> MEEPEEPADSGQSLVPVYIYSPEYVSMCDSLAKIPKRASMVHSLIEAYALHKQMRIVKPKVASMEEMATFHTDAYLQHLQKVSQEGDDDHPDSIEYGLGYDCPATEGIFDYAAAIGGATI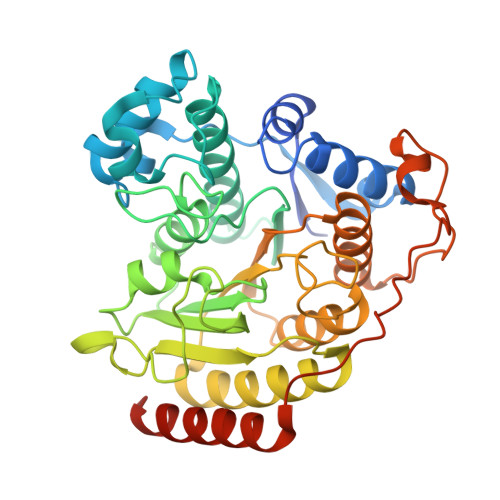TAAQCLIDGMCKVAINWSGGWHHAKKDEASGFCYLNDAVLGILRLRRKFERILYVDLDLHHGDGVEDAFSFTSKVMTVSLHKFSPGFFPGTGDVSDVGLGKGRYYSVNVPIQDGIQDEKYYQICESVLKEVYQAFNPKAVVLQLGADTIAGDPMCSFNMTPVGIGKCLKYILQWQLATLILGGGGFNLANTARCWTYLTGVILGKTLSSEIPDHEFFTAYGPDYVLEITPSCRPDRNEPHRIQQILNYIKGNLKHVVIEGRSHHHHHH Nora virus is a positive-sense, single-stranded RNA virus infecting different Drosophila species including Drosophila melanogaster and Drosophila simulans. Nora virus ORF4, situated at the 3′-terminal end of the genome, encodes a 931 amino acid-long polyprotein. The translated polyprotein is cleaved at two positions (264 aa and 515 aa) post-translationally by a virus-encoded protease to form the virion’s mature structural proteins VP4A (29 kDa), VP4B (28 kDa) and VP4C (48 kDa). The Nora virus capsid asymmetric unit is built from three subunits, a single copy each of VP4A, VP4B and VP4C.

We determined a 2.7 Å resolution Nora virus structure using electron cryo-microscopy and single particle image analysis. The models of capsid proteins VP4A, VP4B and VP4C were built de novo to generate an atomic model of Nora virus constrained by the density from the reconstruction. The Nora virus reconstruction displays an icosahedrally- symmetric particle with a T = 1 (pseudo T = 3) triangulation number; a capsid architecture previously described as one of the main characteristics of the order Picornavirales. Major domains of all the three subunits are β-sheet jelly rolls. The five-fold vertices are composed of VP4C, the three-fold facets are composed of VP4A and VP4B and the two-fold edges are composed of VP4A. We were unambiguously able to trace the C-α backbone for VP4A (residues 1–249 out of 264), for VP4B (2–242 out of 251) and for VP4C (1–364 out of 416). The disordered C-termini regions are presumably exposed on the capsid surface, as the last visible residues contribute to the striking protrusions that circle the pentamers composed of both the VP4B and the VP4C C-termini. However, the most prominent capsid surface features are the 60 mainly α-helical protrusions that are situated at the interface between VP4C contributing most of the residues and VP4B contributing one α-helix. Annulus formation is a primary requirement for intra-pentamer stability in those capsids. It is fulfilled in Nora virus by extensive interaction of VP4B and VP4C N-termini around the five-fold but at a much greater distance from the five-fold axis of symmetry. However, unlike HPeVs, there is a crossover of the VP4A N-terminus (residues 1–13) with a symmetry-equivalent N-terminus of another VP4A from the neighbouring pentamer at the two-fold axis. The symmetry-related, positively-charged histidines (residue number 9) of the two VP4A N-termini on the two-fold axis closely interact with the ssRNA genome.

> SLPENAPNAVSNPQQFITPATALSAEEYNVHEALGETEELELDEFPVLVFKGNVPVDSVTSIPLDLATIYDFAWDGEQNAISQKFQRFAHLIPKSAGGFGPVIGNYTITANLPTGVAGRILHNCLPGDCVDLAVSRIFGLKSLLGVAGTAVSAIGGPLLNGLVNTAAPILSGAAHAIGGNVVGGLADAVIDIGSNLLTPKEKEQPSANSSAISGDIPISRFVEMLKYVKENYQDNPVFPTLLVEPQNFISNAMTALKTIPIEVFANMRNVKVERNLFDRTVVPTVKEATLADIVIPNHMYGYILRDFLQNKRAFQSGTKQNVYFQQFLTVLSQRNIRTHITLNDITSCSIDSESIANKIERVKHYLSTNSSGETTEEFSRTDTGLLPITTRKIVLGESKRRTERYVAETVFPSVRQ;> ADNEVTAEGGKLVQELVYDHSAIPVAPVVETQAEQPEVPVSLVATRKNDTGHLATKWYDFAKISLSNPANMNWTTLTIDPYNNVTLSRDGESMVLPWRRNVWTTGSKSIGYIRTMVAQINIPRPPQISGVLEVKDSINNSSISLVEFGGKVEIPIIPKVMNGLATTASLPRHRLNPWMRTAESKVELQYRIIAFNRTSDIADLNVSVLLRPGDSQFQLPMKPDNNVDTRHFELVEALMYHYDSLRIRGEEQ;> MQNPTQTMHIYDMPLRVIAGLSTLAKTTEEDDNTSTGIVVSEVGEPQVVNHPAWIDPFVAYQLRAPRKNITPDFIFGRADIGNAFSAFLPRRFSAPAVGTRLVVDPVFTYQQRTVLGLYNYFHADFYYIVHVPAPLGTGIYLKIYAPEFDTTTVTRGIRFKPSASPTIALSVPWSNDLSTVETSVGRVGQSGGSIVIETIEDNSNETVNTPLSITVWCCMANIKATGYRHADTSAYNEKGMNFIPVPVPKPPVPPTKPITGEEQ> GHMSGRGKKPTRTLVMTSMPSEKQNVVIQVVDKLKGFSIAPDVCETTTHVLSGKPLRTLNVLLGIARGCWVLSYDWVLWSLELGHWISEEPFELSHHFP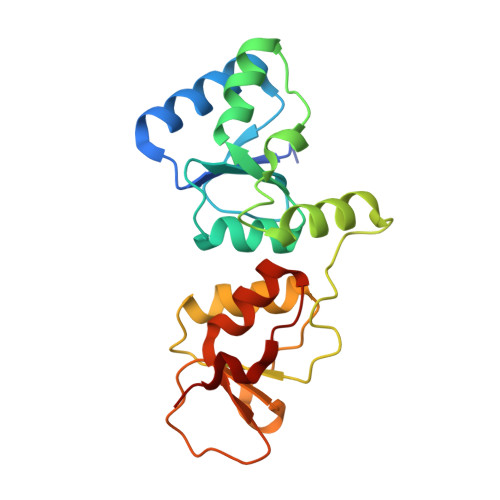AAPLCRSECHLSAGPYRGTLFADQPVMFVSPASSPPVAKLCELVHLCGGRVSQVPRQASIVIGPYSGKKKATVKYLSEKWVLDSITQHKVCAPENYLLSQ>GPGSSHWTSKVHESVIGRNPEGQLGFELKGGAENGQFPYLGEVKPGKVAYESG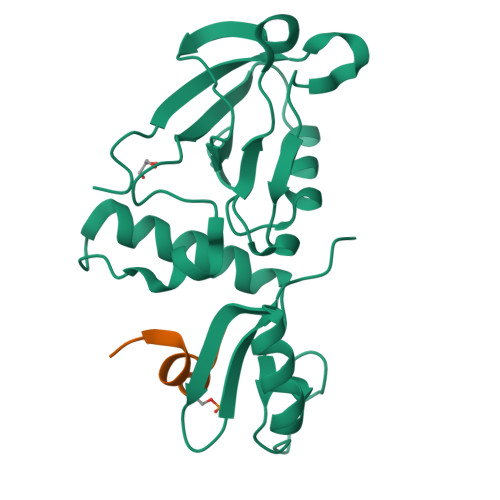SKLVSEELLLEVNETPVAGLTIRDVLAVIKHCKDPLRLKCVKQGGIVDKDLRHYLNLRFQKGSVDHELQQIIRDNLYLRTVPCTTRPHKEGEVPGVDYIFITVEEFMELEKSGALLESGTYEDNYYGTPKPPAEPAPLLNVTDQILPGATPSAEGKRKRNKSVTNMEKASIEPPEEEEEER[2x];>ARRESYLKATQPSL[2x]> GAGCACCTGTA;> ACACCGT;> TCTGACTGTGGTGC;> ACGGACAGT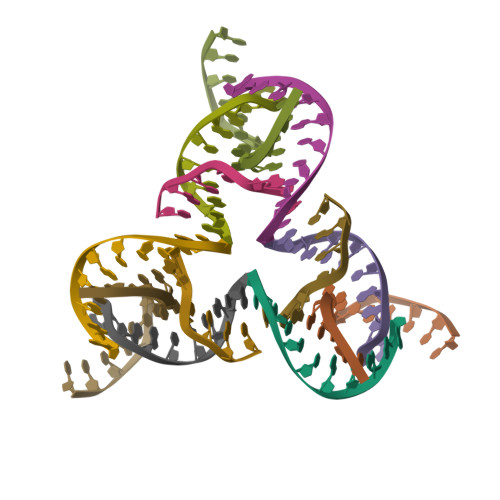CA> FNELS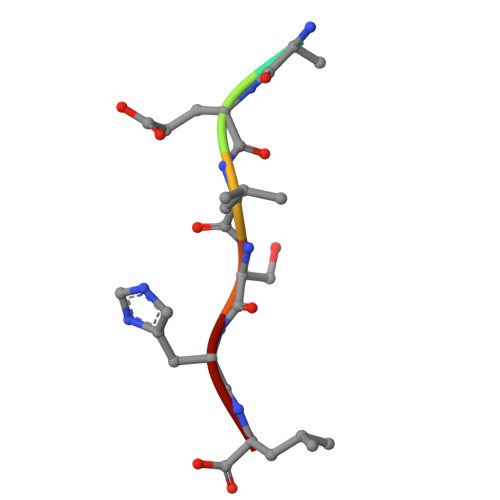HL> MKHQHQHQHQHQHQQPLQEEEQAHATSLPPRASSPPQILPQLSPEQLGMIEKLVAAQQQCNRRSFSDRLRVTPWPMAPDPHSREARQQRFAHFTELAIVSVQEIVDFAKQLPGFLQLSREDQIALLKTSAIEVMLLETSRRYNPGSESITFLKDFSYNREDFAKAGLQVEFINPIF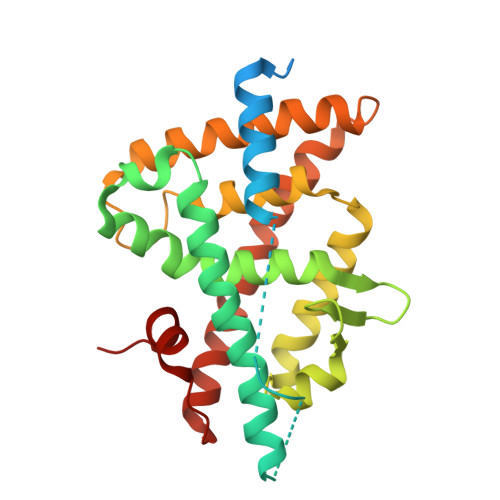EFSRAMNELQLNDAEFALLIAISIFSADRPNVQDQLQVERLQHTYVEALHAYVSIHHPHDRLMFPRMLMKLVSLRTLSSVHSEQVFALRLQDKKLPPLLSEIWDVHE>[2x]MPVTINNFNYNDPIDNNNIIMMEPPFARGTGRYYKAFKITDRIWIIPERYTFGYKPEDFNKSSGIFNRDVCEYYDPDYLNTNDKKNIFLQTMIKLFNRIKSKPLGEKLLEMIINGIPYLGDRRVPLEEFNTNIASVTVNKLISNPGEVERKKGIFANLIIFGPGPVLNENETIDIGIQNHFASREGFGGIMQMKFCPEYVSVFNNVQENKGASIFNRRGYFSDPALILMHQLIYVLHGLYGIKVDDLPIVPNEKKFFMQSTDAIQAEELYTFGGQDPSIITPSTDKSIYDKVLQNFRGIVDRLNKVLVCISDPNININIYKNKFKDKYKFVEDSEGKYSIDVESFDKLYKSLMFGFTETNIAENYKIKTRASYFSDSLPPVKIKNLLDNEIYTIEEGFNISDKDMEKEYRGQNKAINKQAYEEISKEHLAVYKIQMCKSVKAPGICIDVDNEDLFFIADKNSFSDDLSKNERIEYNTQSNYIENDFPINELILDTDLISKIELPSENTESLTDFNVDVPVYEKQPAIKKIFTDENTIFQYLYSQTFPLDIRDISLTSSFDDALLFSNKVYSFFSMDYIKTANKVVEAGLFAGWVKQIVNDFVIEANKSNTMDKIADISLIVPYIGLALNVGNETAKGNFENAFEIAGASILLEFIPELLIPVVGAFLLESYIDNKNKIIKTIDNALTKRNEKWSDMYGLIVAQWLSTVNTQFYTIKEGMYKALNYQAQALEEIIKYRYNIYSEKEKSNINIDFNDINSKLNEGINQAIDNINNFINGCSVSYLMKKMIPLAVEKLLDFDNTLKKNLLNYIDENKLYLIGSAEYEKSKVNKYLKTIMPFDLSIYTNDTILIEMFNKYNSEILNNIILNLRYKDNNLIDLSGYGAKVEVYDGVELNDKNQFKLTSSANSKIRVTQNQNIIFNSVFLDFSVSFWIRIPKYKNDGIQNYIHNEYTIINCMKNNS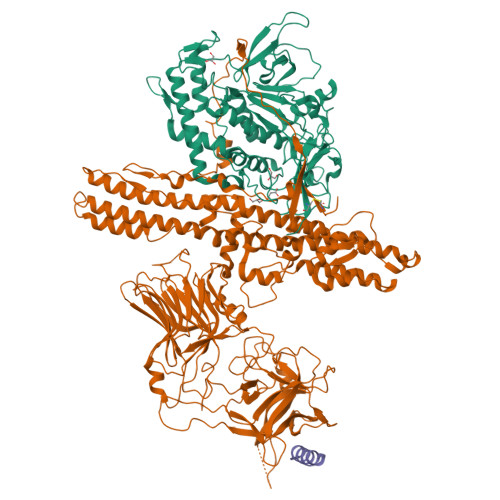GWKISIRGNRIIWTLIDINGKTKSVFFEYNIREDISEYINRWFFVTITNNLNNAKIYINGKLESNTDIKDIREVIANGEIIFKLDGDIDRTQFIWMKYFSIFNTELSQSNIEERYKIQSYSEYLKDFWGNPLMYNKEYYMFNAGNKNSYIKLKKDSPVGEILTRSKYNQNSKYINYRDLYIGEKFIIRRKSNSQSINDDIVRKEDYIYLDFFNLNQEWRVYTYKYFKKEEMKLFLAPIYDSDEFYNTIQIKEYDEQPTYSCQLLFKKDEESTDEIGLIGIHRFYESGIVFEEYKDYFCISKWYLKEVKRKPYNLKLGCNWQFIPKDEGWTE;> GEGKEDAFSKLKEKFMNELHK> AEAGITGTWYAQLGDTFIVTAGADGALTGTYEAAVGNAESRYVLTGRYDSAPATDGSGTALGWTVAWKNNYRNAHSATTWSGQYVGGAEARINTQWLLTSGTTEANAWKSTLVGHDTFTKVKPSAASA;> AEAGITGTWYNQLGSTFIVTAGADGALTGTYESAVGNAESRYVLTGRYDSAPATDGSGTALGWTVAWKNNYRNAHSATTWSGQYVGGAEARINTQWLLTSGTTEANAWKSTLVGHDTFTKVKPSAASEEEEEE

The femtomolar affinity of streptavidin/avidin for biotinylated targets, combined with resilience to harsh conditions and an on-rate of ~ 107 M− 1 s− 1, is the basis for biotin's central role as a specific biological “glue” in diverse research methods and biotechnologies. We previously generated streptavidin heterotetramers with exactly one, two, or three functional biotin-binding sites, through purifying tetramers containing defined numbers of non-biotin-binding “Dead” and His6-tagged wild-type subunits. However, tetramers with two functional and two Dead subunits can assemble in three different arrangements. To generate a controlled and stable bridge for bionanotechnology, we demonstrate here a method for the simple isolation of streptavidin variants with precise cis-divalent or 1,3 trans-divalent arrangements.

To understand interaction between ligand binding sites, we solved 1,3 trans-divalent streptavidin's crystal structure bound to biotin-4-fluorescein. Biotin-4-fluorescein represents the largest ligand where there is a crystal structure with streptavidin or avidin, as well as a widely used probe of the binding kinetics and capacity of biotin-binding proteins. Our 2.3-Å-resolution structure shows the 1,4 dimer in the asymmetric unit (one copy of SAe and one copy of D). Building the native streptavidin tetramer from this dimer shows that the two biotin-4-fluorescein molecules are in the expected trans arrangement. All the contacts of the 1,3 trans-divalent streptavidin with the biotin moiety are as expected. Fluorescein and the ethylene diamine spacer form several non-polar contacts to streptavidin not observed with biotin. Trp120 is 5 Å from fluorescein and may explain part of the quenching of fluorescence. Biotin-4-fluorescein bound in chain b reaches over and interacts with residues of chain d. However, we do not believe this conformation of biotin-4-fluorescein is the same as when four ligands are bound to the same tetramer: if the SAe:biotin-4-fluorescein complex were in a cis arrangement, there would be an obvious clash between the fluorescein moieties of neighboring ligands. Even with a ligand as small as biotin-4-fluorescein, our structure showed the interactions that would inhibit cis binding.Cation-chloride cotransporters (CCC) are central to the regulation of intracellular Cl− concentration and have key physiological roles in neuronal excitability, trans-epithelial salt and water movement, and regulation of cell volume. The CCCs are strictly electroneutral transporters, NKCCs transporting two Cl− ions coupled to the movement of one Na+ and one K+, whereas NCC and KCC couple the movement of one Cl− ion and either Na+ or K+ respectively. All CCCs are feedback-regulated by the concentration of intracellular Cl−—this is mediated by the WNK (kinase with no lysine)-SPAK/OSR1 (SPS1-related proline/alanine-rich kinase/oxidative stress-responsive kinase 1) signaling pathway. Here, using single-particle cryo-electron microscopy (cryo-EM), we report the structures of human NKCC1 (hNKCC1a) and mouse KCC2 (mKCC2a) at 3.5 and 3.8 Å resolution, respectively.

The mKCC2 structure is in a similar inward-open inactive state but with an inhibitory N-terminus peptide in place to block the translocation pore, and with a very different dimer architecture compared to KCC1—together these exciting structures allow us to propose models for the regulatory mechanisms of CCCs and to gain insight into the defects in known human mutations. In the case of mKCC2, using mass spectrometry we confirmed phosphorylation at the two sites in the C terminus (T929 and T1029) whose phosphorylation appears necessary and possibly sufficient to inactivate KCC transport function; additional evidence will be seen below from the blocked pore in the mKCC2 structure. Within the TM region of mKCC2, we noted a helix-loop density that we were able to assign to residues 85–108 in the N terminus, lying in a cleft between TMs 1, 5, 6, and 8. Residues T92 and Q96 from the N terminus interact with R443 and S444 from TM6b, while the additional N-terminus residues N93 and E102 interact with Q524 and R538 from TM8. The presence of this bound N-terminus peptide is a marked finding since at this position it is expected to completely inhibit function: in addition to the inhibitory interactions with critical TMs 6 and 8, the peptide completely blocks access to the otherwise-inward-open pore. Compared with wild-type mKCC2, a mutant with deletion of residues 85–120 in the N terminus was found to have increased transporter activity, strongly supporting an inhibitory role of this N-terminal region in KCC transporters. At the extracellular end, E224 from TM3 interacts with R142 from TM1b to prevent access from the extracellular side congruent with the apparent gate in hKCC139 and above in hNKCC1. Furthermore, analogous to the intracellular essential residues of hNKCC1, R193 from ICL1 of mKCC2 is close to D539 in TM8, forming a polar interaction, and from sequence conservation, it appears that all the CCC transporters utilize this interaction.

>MSRRFTVTSLPPAASAASADPESRRHSVADPRRLPREDVKGDGNPKESSPFINSTDTEKGREYDGRNMALFEEEMDTSPMVSSLLSGLANYTNLPQGSREHEEAENNEGGKKKPVQAPRMGTFMGVYLPCLQNIFGVILFLRLTWVVGIAGIMESFCMVFICCSCTMLTAISMSAIATNGVVPAGGSYYMISRSLGPEFGGAVGLCFYLGTTFAGAMYILGTIEILLAYLFPAMAIFKAEDASGEAAAMLNNMRVYGTCVLTCMATVVFVGVKYVNKFALVFLGCVILSILAIYAGVIKSAFDPPNFPICLLGNRTLSRHGFDVCAKLAWEGNETVTTRLWGLFCSSRLLNATCDEYFTRNNVTEIQGIPGAASGLIKENLWSSYLTKGVIVERRGMPSVGLADGTPVDMDHPYVFSDMTSYFTLLVGIYFPSVTGIMAGSNRSGDLRDAQKSIPTGTILAIATTSAVYISSVVLFGACIEGVVLRDKFGEAVNGNLVVGTLAWPSPWVIVIGSFFSTCGAGLQSLTGAPRLLQAISRDGIVPFLQVFGHGKANGEPTWALLLTACICEIGILIASLDEVAPILSMFFLMCYMFVNLACAVQTLLRTPNWRPRFRYYHWTLSFLGMSLCLALMFICSWYYALVAMLIAGLIYKYIEYRGAEKEWGDGIRGLSLSAARYALLRLEEGPPHTKNWRPQLLVLVRVDQDQNVVHPQLLSLTSQLKAGKGLTIVGSVLEGTFLDNHPQAQRAEESIRRLMEAEKVKGFCQVVISSNLRDGVSHLIQSGGLGGLQHNTVLVGWPRNWRQKEDHQTWRNFIELVRETTAGHLALLVTKNVSMFPGNPERFSEGSIDVWWIVHDGGMLMLLPFLLRHHKVWRKCKMRIFTVAQMDDNSIQMKKDLTTFLYHLRITAEVEVVEMHESDISAYTYEKTLVMEQRSQILKQMHLTKNEREREIQSITDESRGSIRRKNPANPRLRLNVPEETACDNEEKPEEEVQLIHDQSAPSCPSSSPSPGEEPEGERETDPEVHLTWTKDKSVAEKNKGPSPVSSEGIKDFFSMKPEWENLNQSNVRRMHTAVRLNEVIVNKSRDAKLVLLNMPGPPRNRNGDENYMEFLEVLTEQLDRVMLVRGGGREVITIYS[2x]> MNYTETVAYIHSFPRLAKTGDHRRILTLLHALGNPQQQGRYIHVTGTNGKSSAANAIAHVLEASGLTVGLYTSPFIMRFNERIMI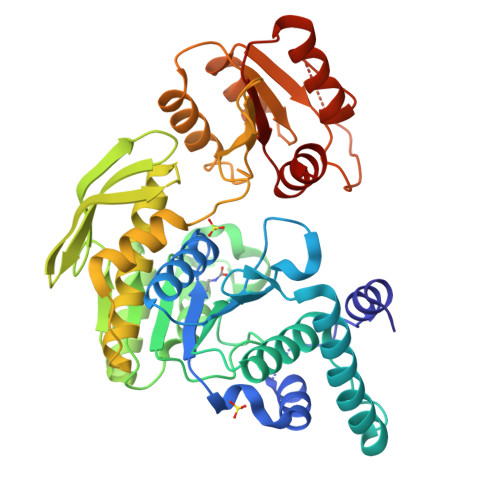DHEPIPDAALVNAVAFVRAALERLQQQQADFNVTEFEFITALGYWYFRQRQVDVAVIEVGIGGDTDSTNVITPVVSVLTEVALDHQKLLGHTITAIAKHKAGIIKRGIPVVTGNLVPDAAAVVAAKVATTGSQWLRFDRDFSVPKAKLHGWGQRFTYEDQDGRISDLEVPLVGDYQQRNMAIAIQTAKVYAKQTEWPLTPQNIRQGLAASHWPARLEKISDTPLIVIDGAHNPDGINGLITALKQLFSQPITVIAGILADKDYAAMADRLTAAFSTVYLVPVPGTPRALPEAGYEALHEGRLKDSWQEALAASLNDVPDQPIVITGSLYLASAVRQTLLGGKS Here, we identified the BBDE_2040 gene product from Bifidobacterium dentium (α-D-fructofuranosidase and difructose dianhydride I synthase/hydrolase from Bifidobacterium dentium [αFFase1]) as an enzyme with α-D-fructofuranosidase and α-D-arabinofuranosidase activities and an anomer-retaining manner. αFFase1 is not homologous with any known enzymes, suggesting that it is a member of a novel glycoside hydrolase family. αFFase1 did not catalyze any reactions when DFA III or inulin was used as a substrate, and there were no significant peak changes in the reaction of caramelized sugars other than those of the four peaks. These results indicate that αFFase1 specifically catalyzes the reversible hydrolysis of the intramolecular α-(2→1′)-D-fructofuranosidic bond of DFA I and DHL II. Because of the significant bias of equilibrium toward DFA synthesis, we propose a common name difructose dianhydride I synthase/hydrolase for this enzyme (EC 3.2.1.134). Each monomer consists of β-jelly roll 1 (residues 3–200, green), β-jelly roll 2 (201–396, magenta), and a 51-amino acid–long α-helix at the C terminus (397–448, blue), englobing the whole structure.

The structures of αFFase1 complexed with D-fructose and D-arabinose were determined at a resolution of 1.76 and 1.87 Å, respectively. In the active sites of all six chains, β-Fruf and β-Araf were observed in similar conformations at the expected −1 subsite. The furanose ring of β-Fruf and β-Araf adopts E5 (P ∼ 35°) and 3T4 (P ∼ 54°) conformations, respectively, as analyzed by the Altona–Sundaralingam phase angle parameter. These conformations correspond to the “northeast” conformation of the pseudorotational map. The sugar ligands are surrounded by Trp267, Glu270, Glu291, Asp292, Trp298, and Tyr187′ (prime indicates that this residue is from the neighboring protomer). Notably, Glu291 and Glu270 are positioned close to the anomeric C2 atom from the β and α configuration sides, respectively. Therefore, Glu291 and Glu270 are suggested to be nucleophile and acid/base catalyst residues, respectively. The Ca2+ is coordinated by the side chains of Asn31′, Asp33′, and Asn272, the main chain carbonyl of Glu270 and Thr288, and two water molecules. One of the two coordinating water molecules forms a hydrogen bond with the C4 hydroxy group of Fruf (C3 hydroxy of Araf).

>[6x]MSEITGLFKDLTKVKHARNGRLASWDQRGKNQDYWEIPAGESITLGEIEGPGCITHMWMTSSCRKVVAPSILDPELNASAAPVMEIHPALGVIWDAYDPFYYRKALIKITWDDQDTPSVLVPFGDFFCIGNSYPGNFSSLPFNVSLKPEEAGKFGAPCSVSCYFPMPFNKKAKIEIVNDNELPFILYFNIDYEMYGEPLPEDTAYFHAAWHRENPCNGWGPELQVNSPEVNNVTNFKGENNYTVLDVEGTGHYVGCNLTVKHFQGSWWGEGNDMFFIDGEEYPSLNGTGTEDYFNHAWGMQRNAYPFFGTIVHEGDTDGFQVSYRWHITDPVRFEKHLKVTIEHGHANQLSDDWSSTAYWYQILPTASRITIAPVEDRLPVVPQLPERKLVLPQLTEEQQAARDTYQKRWKDYEPRRDTQFRIKEDKARRESKLNTEFAKKLRDAFDAEREQLEHHHHHH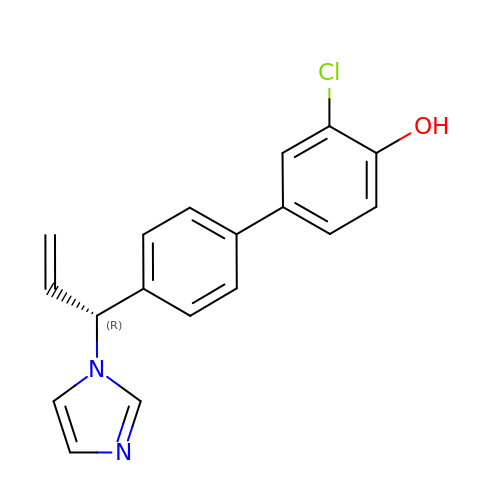2-chloranyl-4-[4-[(1~{R})-1-imidazol-1-ylprop-2-enyl]phenyl]phenol | C18 H15 Cl N2 O | BOCKNSHTLMSFKF-QGZVFWFLSA-N>[2x]MGSSHHHHHHSQDPMSLNLVSEQLLAANGLKHQDLFAILGQLAERRLDYGDLYFQSSYHESWVLEDRIIKDGSYNIDQGVGVRAISGEKTGFAYADQISLLALEQSAQAARTIVRDSGDGKVQTLGAVEHSPLYTSVDPLQSMSREEKLDILRRVDKVAREADKRVQEVTASLSGVYELILVAATDGTLAADVRPLVRLSVSVLVEEDGKRERGASGGGGRFGYEFFLADLDGEVRADAWAKEAVRMALVNLSAVAAPAGTMPVVLGAGWPGVLLAEAVGHGLEGDFNRRGTSVFSGQVGELVASELCTVVDDGTMVDRRGSVAIDDEGTPGQYNVLIENGILKGYMQDKLNARLMGMTPTGNGRRESYAHLPMPRMTNTYMLPGKSTPQEIIESVEYGIYAPNFGGGQVDITSDKFVFSTSEAYLIENGKVTKPVKGATLIGSGIETMQQISMVGNDLKLDNGVGVCGKEGQSLPVGVGQPTLKVDNLTVGGTA;>[2x]MALAMKVISQVEAQRKILEEAVSTALELASGKSDGAEVAVSKTTGISVSTRYGEVENVEFNSDGALGITVYHQNRKGSASSTDLSPQAIARTVQAALDIARYTSPDPCAGVADKELLAFDAPDLDLFHPAEVSPDEAIELAARAEQAALQADKRITNTEGGSFNSHYGVKVFGNSHGMLQGYCSTRHSLSSCVIAEENGDMERDYAYTIGRAMSDLQTPEWVGADCARRTLSRLSPRKLSTMKAPVIFANEVATGLFGHLVGAIAGGSVYRKSTFLLDSLGKQILPDWLTIEEHPHLLKGLASTPFDSEGVRTERRDIIKDGILTQWLLTSYSARKLGLKSTGHAGGIHNWRIAGQGLSFEQMLKEMGTGLVVTELMGQGVSAITGDYSRGAAGFWVENGEIQYPVSEITIAGNLKDMWRNIVTVGNDIETRSNIQCGSVLLPEMKIAGQ;>AAAAA[2x]

Using a combination of biochemical and crystallographic methods we show that E. coli TldD and TldE interact to form a heterodimeric metalloprotease. TldD/E cleaves the N-terminal leader sequence from the modified MccB17 precursor peptide, to yield mature antibiotic, while it has no effect on the unmodified peptide. Both proteins are essential for the activity; however, only the TldD subunit forms a novel metal-containing active site within the hollow core of the heterodimer. Peptide substrates are bound in a sequence-independent manner through β sheet interactions with TldD and are likely cleaved via a thermolysin-type mechanism.

We have constructed His262 and His267 alanine substitution mutants, of which His267Ala was not folded correctly and His262Ala was catalytically inactive but, surprisingly, had wild-type Zn/Fe content as determined by ICP-AES. a We have used a two-part dataset naming convention comprising the TldD variant type (WT, wild-type), plus a shorthand for the ligand bound at the active site, where PO4, phosphate; DRVY and HPF, sequences of angiotensin fragments; Act, actinonin; hex and pent, adventitiously bound hexa- and pentapeptides. N.B.: details of the H262A-pent structure are found in Figure S7. H262A-pent peptide ligand was refined with occupancy of 0.5.Proliferating cell nuclear antigen (PCNA) is a protein that is essential for many DNA metabolic processes including DNA replication, base excision repair, nucleotide excision repair, mismatch repair, and recombination. PCNA is a ring-shaped homo-trimer that acts as a sliding clamp that encircles DNA forming a scaffold for binding numerous proteins involved in DNA metabolism. PCNA is required for translesion synthesis (TLS), which is a pathway for bypassing DNA damage during replication. The subunit interface of PCNA is comprised of two anti-parallel β strands: strand I1 (residues 109 to 117) in domain 1 of one subunit and strand D2 (residues 175 to 183) in domain 2 of the adjacent subunit.

To better understand the role of the subunit interface in translesion synthesis and in other DNA metabolic processes, we used random mutagenesis to generate a series of PCNA mutant proteins with substitutions in either of these two β strands. We first measured the growth rate of these 17 strains in liquid media. Twelve of these strains (A112G, Y114F, S115E, S115G, S115V, S177G, S177L, S177V, G178L, G178M, S178T, and V180A) had slower growth rates than the wild type strain of approximately 4 to 5 hours. The Y114F, S115V, and V180A mutants, which had a slower growth rate in this assay, showed no growth defect in the spotting assay. We next measured the UV sensitivity of these 17 strains. Six of these strains (Y114A, Y114F, S115E, G178L, V180A, and I181R) had the same increased level of UV sensitivity as the K164R control strain. We then examined the rates of spontaneous mutagenesis and the rates of UV-induced mutagenesis of these 17 strains as well as E113G and G178S. The E113G, Y114A, and G178M strains had an approximately two-fold increase in the rate of spontaneous mutagenesis, while the S115E and V180A strains had an approximately 4-fold increase. By contrast, all 17 strains, except the S177G, S179A, and V180A mutant strains, had statistically significant defects in the rate of UV-induced mutagenesis (with p values less than 0.05). A defect in UV-induced mutagenesis is a characteristic indicator of a defect in error-prone TLS.

> HMLEAKFEEASLFKRIIDGFKDCVQLVNFQCKEDGIIAQAVDDSRVLLVSLEIGVEAFQEYRCDHPVTLGMDLTSLSKILRCGNNTDTLTLIADNTPDSIILLFEDTKKDRIAEYSLKLMDIDADFLKIEELQYDSTLSLPSSEFSKIVRDLSQLSDSINIMITKETIKFVADGDIGSGSAIIKPFVDMEHPETSIKLEMDQPVDLTFGAKYLLDIIKGSSLSDRVGIRLSSEAPALFQFDLKSGFLQFFLAPKFNDEE> MGHHHHHHMKSGRGKKPTRTLVMTSMPSEKQNVVIQVVDKLKGFSIAPDVCETTTHVLSGKPLRTLNVLLGIARGCWVLSYDWVLWSLELGHWISEEPFELSHHFPAAPLC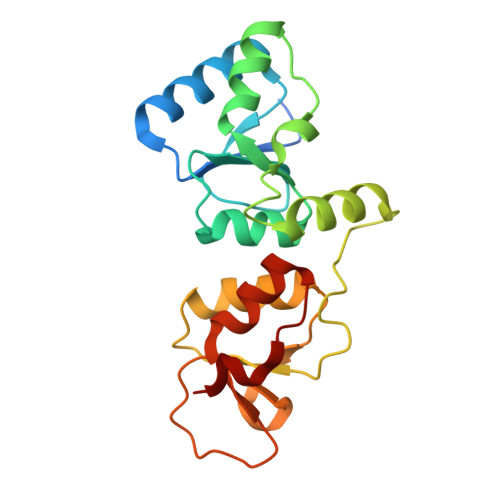RSECHLSAGPYRGTLFADQPAMFVSPASSPPVAKLCELVHLCGGRVSQVPRQASIVIGPYSGKKKATVKYLSEKWVLDSITQHKVCAPENYLLSQ>[3x]GSMKKVEAIIRPEKLEIVKKALSDAGYVGMTVSEVKGRGV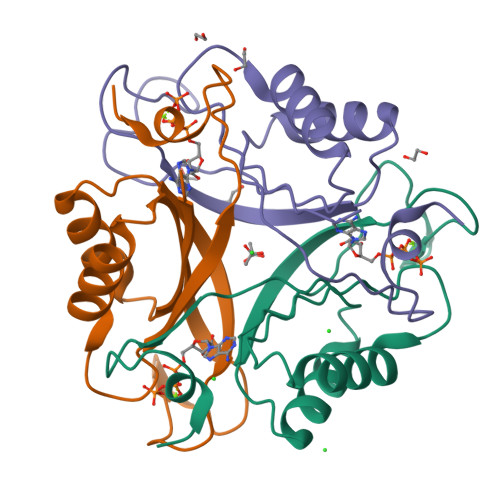QGGIVERYRGREYIVDLIPKVKIELVVKEEDVDNVIDIICENARTGNPGDGKIFVIPVERVVRVRTKEEGKEALLEHHH>GSHMISEHDSVLEKYPRIQKVLNSTVPALSLNSSTRYEGKIINIGGTIIKARLPKARIGAFYKIEPSQRLAEVIAIDEDEVFLLPFEHVSGMYCGQWLSYQGDEFKIRVGDALLGRLIDGIGRPMESNIVAPYLPFERSLYAEPPDPLLRQVIDQPFILGVRAIDGLLTCGIGQRIGIFAGSGVGKSTLLGMICNGASADIIVLALIGERGREVNEFLALLPQSTLSKCVLVVTTSDRPALERMKAAFTATTIAEYFRDQGKNVLLMMDSVTRYARAARDVGLASGEPDVRGGFPPSVFSSLPKLLERAGPAPKGSITAIYTVLLESDNVNDPIGDEVRSILDGHIVLTRELAEENHFPAIDIGLSASRVMHNVVTSEHLRAAAECKKLIATYKNVELLIRIGEYTMGQDPEADKAIKNRKLIQNFIQQSTKDISSYEKTIESLFKVVA[6x];> GSHMLDRILSIRKSRANRLRESMAKINSQIKEVDGKLDDCEQSIKESIASKQAYCASLVNLDKVSLYKYQIKNNAFDEQKQRLYEKKSSLSKEKRSLLDSQKRTKENLQHVNKSVEKLSFAIKEHYFD

Substrate selection occurs in the cytoplasm and inner membrane, mediated by the export gate subcomplex (EscRSTUV in EPEC, and FliPQR, FlhB, FlhA in flagella) and the cytoplasmic ATPase complex (ATPase EscN, peripheral stalk EscL, and central stalk EscO; flagellar FliI, FliH and FliJ, respectively). The T3SS ATPase homologues are made distinct by their homohexameric construction, a presumed ancestral precursor to the heterohexameric rotary F1/V1-ATPases. The ATPase has been proposed to specifically enhance PMF-induced secretion efficiency, as well as to play a role in effector targeting, release from chaperones and unfolding prior to secretion. Each EscN monomer displays three sub-domains: the N-terminal oligomerization domain (residues 1–102), a cluster of curved β-sheets; the ATPase domain (103–372), made up of a central Rossmann fold with seven parallel β-strands flanked by four α-helices on one side and three on the other; and the C-terminal domain (373–446), made up of four helices lining the central pore.

The EscN-EscO complex was subjected to single-particle cryo-EM, with 3D classification resulting in two primary classes that refined to high resolution. Class 1 (58,000 particles, 3.34 Å) reveals a homohexameric EscN pore lacking visible EscO density, while class 2 (55,000 particles, 3.29 Å) looks similar but with additional α-helical density for approximately half of a single EscO molecule resolved. The EscN model remained similar when refined into the class 2 map (Cα root-mean-square deviation (RMSD) of ~0.5 Å over 2130 residues), with unfilled density from two associated anti-parallel helices attributed to EscO. The quality of the side-chain density was sufficient for sequence assignment of EscO residues 0 (from affinity tag) to 30 and 91 to 122 out of a total of 125 residues. Extending the structural and functional similarity to the rotary ATPases, both the N- and C-termini of the EscO coiled coil are observed to penetrate the EscN C-terminal pore opening. In contrast to the F1- and V1-ATPase complexes where the central stalk subunit extends ~70 Å into the catalytic core, EscO only penetrates ~30 Å, preventing interaction with all but the C-terminal domains. The two resolved helices of EscO are bound in a semicircle formed by the same EscN helix-loop region (residues Leu395–Glu401) from chains NA through NE, which congregate along one-half of the pore due to EscN’s tilt; this region in chain NF, the most loosely packed chain, is directly opposite the bound EscO and poorly ordered. EscN creates a cradle of negative charge provided predominantly by clustered Glu401 from chains NA through NE (conserved in injectisome orthologues and structurally conserved with the F1 β-subunit DELSEED motif), situated on the apex of the pore-proximal loop.(5E)-5-[(N-methoxy-N-methylcarbamimidoyl)imino]-L-norvaline 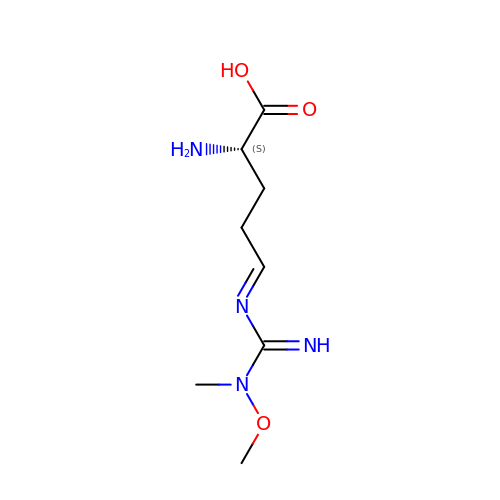| C8 H16 N4 O3 | QNJBMUDCQGTHKO-SOKYQSCGSA-N> MTQPLVGKQILIVEDEQVFRSLLDSWFSSLGATTVLAADGVDALELLGGFTPDLMICPIAMPRMNGLKLLEHIRNRGDQTPVLVISATENMADIAKALRLGVEDVLLKPVKDLNRLREMVFACLYPSMFNSRVEEEERLFRDWDAMVDNPAAAA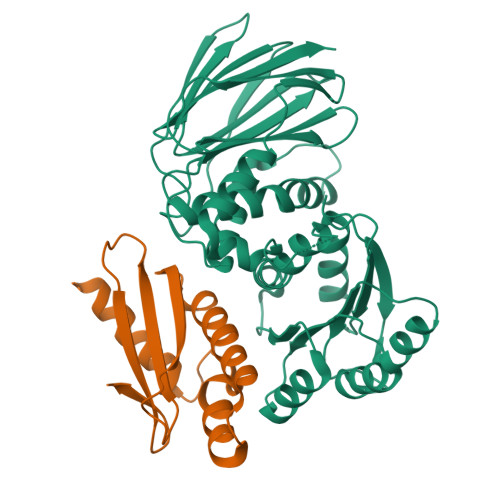KLLQELQPPVQQVISHCRVNYRQLVAADKPGLVLDIAALSENDLAFYCLDVTRAGHNGVLAALLLRALFNGLLQEQLAHQNQRLPELGALLKQVNHLLRQANLPGQFPLLVGYYHRELKNLILVSAGLNATLNTGEHQVQISNGVPLGTLGNAYLNQLSQRCDAWQCQIWGTGGRLRLMLSAE;> MKTSSLRKSVCSDLLTLFNSPHSALPSLLVSGMPEWQVHNPSDKHLQSWYCRQLRSALLFHEPRIAALQVNLKEAYCHTLAISLEIMLYHDDEPLTFDLVWDNGGWRSATLENVS> GAMESKK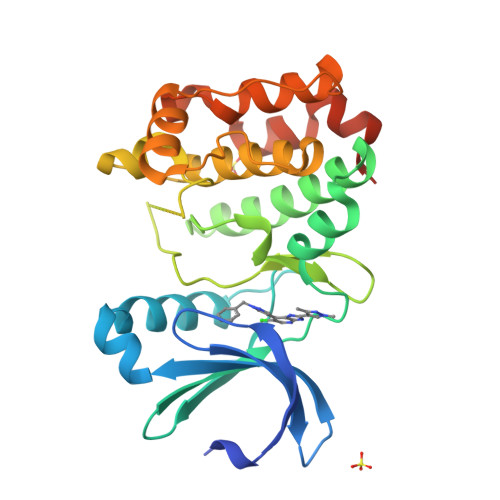RQWALEDFEIGRPLGKGKFGNVYLAREKQSKFILALKVLFKAQLEKAGVEHQLRREVEIQSHLRHPNILRLYGYFHDATRVYLILEYAPLGTVYRELQKLSKFDEQRTATYITELANALSYCHSKRVIHRDIKPENLLLGSAGELKIADFGWSVHAPSSRRTTLAGTLDYLPPEMIEGRMHDEKVDLWSLGVLCYEFLVGKPPFEANTYQETYKRISRVEFTFPDFVTEGARDLISRLLKHNPSQRPMLREVLEHPWITANSSKPSNAQNKESASKQS>TELTKCKVSHAIKDIDGYQGISLLEWACVLFHTSGYDTQAVVNDNGSTEYGLFQISDRFWCKSSEFPESENICGISCDKLLDDELDDDIACAKKILAIKGIDYWKAYKPMCSEKLEQWRCEKP[2x];>ASMTGGQQMGRGSSLTACPEESPLLVGPMLIEFNIPVDLKLVEQQNPKVKLGGRYTPMDCISPHKVAIIIPFRNRQEHLKYWLYYLHPILQRQQLDYGIYVINQAGESMFNKAKLLNVGFKEALKDYDYNCFVFSDVDLIPMNDHNTYRCFSQPRHISVAMDKFGFSLPYVQYFGGVSALSKQQFLSINGFPNNYWGWGGEDDDIYNRLAFRGMSVSRPNAVIGKTRMIRHSRDKKNEPNPQRFDRIAHTKETMLSDGLNSLTYMVLEVQRYP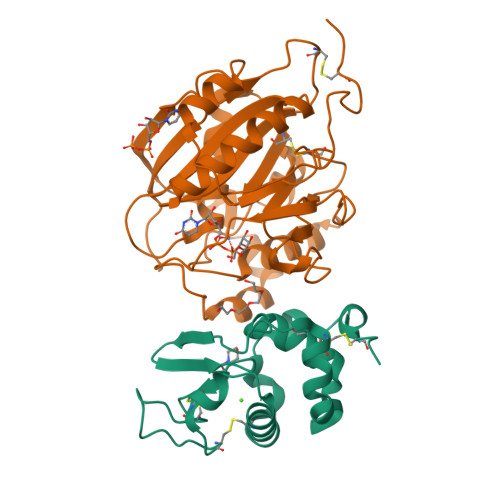LYTKITVDIGTPS[2x]> MTTTERPDLAWLDEVTMTQLERNPYEVYERLRAEAPLAFVPVLGSYVASTAEVCREVATSPDFEAVITPAGGRTFGHPAIIGVNGDIHADLRSMVEPALQPAEVDRWIDDLVRPIARRYLERFENDGHAELVAQYCEPVSVRSLGDLLGLQEVDSDKLREWFAKLNRSLTNAAVDENGEFANPEGFAEGDQAKAEIRAVVDPLIDKWIEHPDDSAISHWLHDGMPPGQTRDREYIYPTIYVYLLGAMQEPGHGMASTLVGLFSRPEQLEEVVDDPTLIPRAIAEGLRWTSPIWSATARISTKPVTIAGVDLPAGTPVMLSYGSANHDTGKYEAPSQYDLHRPPLPHLAFGAGNHACAGIYFANHVMRIALEELFEA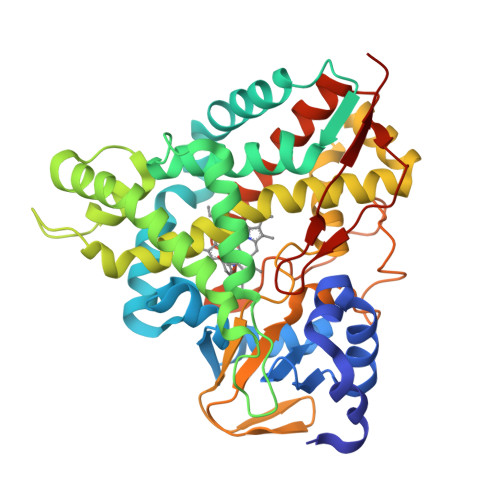IPNLERDTREGVEFWGWGFRGPTSLHVTWEV> MSVGLIAPLASPIQESRANTNIENIGDGAEVIKRTE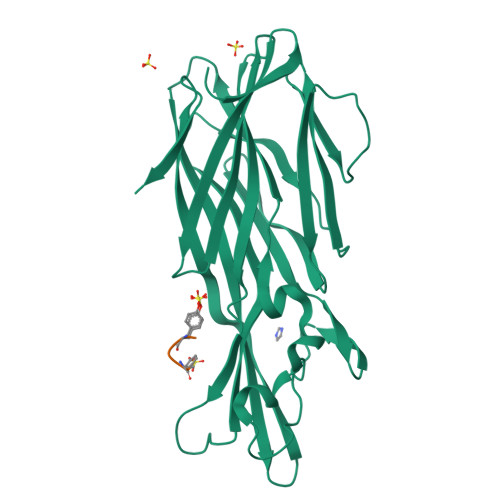DVSSKKWGVTQNVQFDFVKDKKYNKDALIVKMQGFINSRTSFSDVKGSGYELTKRMIWPFQYNIGLTTKDPNVSLINYLPKNKIETTDVGQTLGYNIGGNFQSAPSIGGNGSFNYSKTISYTQKSYVSEVDKQNSKSVKWGVKANEFVTPDGKKSAHDRYLFVQSPNGPTGSAREYFAPDNQLPPLVQSGFNPSFITTLSHEKGSSDTSEFEISYGRNLDITYATLFPRTGIYAERKHNAFVNRNFVVRYEVNWKTHEIKVKGHNKHHHHHH;> XDYDYG> GSAMTVAYIAIGSNLASPLEQVNAALKALGDIPESHILTVSSFYRTPPLGPQDQPDYLNAAVALETSLAPEELLNHTQRIELQQGRVRKAERWGPRTLDLDIMLFGNEVINTERLT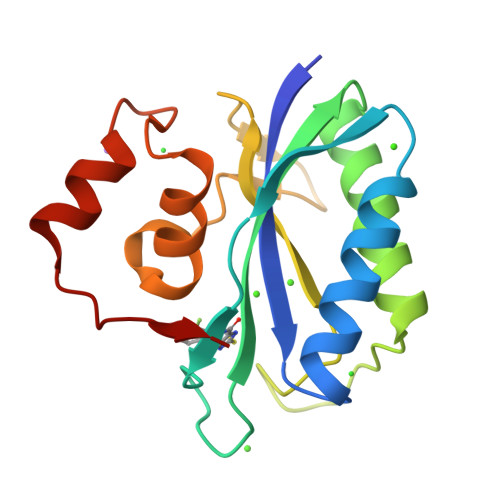VPHYDMKNRGFMLWPLFEIAPELVFPDGEMLRQILHTRAFDKLNKW> GSHMESPKEVLSRVQDAGLTLTNPNDLYWMVDFLKEKYYDNGDYYYPIKTVCDGESIDVKFYCPFEPSLSPHYLELYGSRDERASIYETTMKKYNRINSEKTSAICTPYSSYGDTQIVAYFYSMMYYINDQTAHLKLPESEIESELIDILNDDILIYLNEFMSIFEPEDAQDLERIWDFLDFYQPYFSKVDGKIVLDEKYLVRTPSQMPLIKTICEYVSEQFAPSKNITQVIWEVVRYIKGVKDEIHIRGDKSFTLSLQEYDDFRDKVT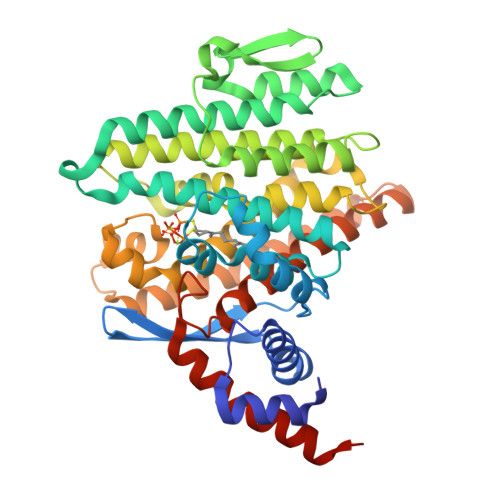ASPMAHAVSDLTHERFSYEAYTNPAFMELENRCSEIITYFNDVCTSDRERLDEDPFNSVFILMDLDPSLNFAKSCDVVVEHAYNKMQAFLKLKEEILESASDEEERLALARMIKTREDSLIGYVLHEVCCVEDGYARDHKPLMKAFLEEEITKSLAEKVKFNPVESESVRLN>GTMAAAAVVAATVPAQSMGADGASSVHWFRKGLRLHDNPALL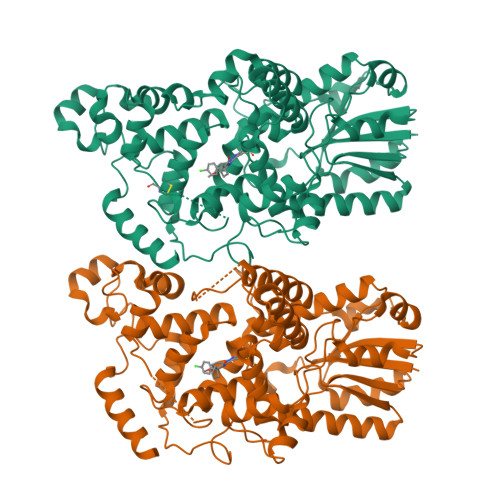AAVRGARCVRCVYILDPWFAASSSVGINRWRFLLQSLEDLDTSLRKLNSRLFVVRGQPADVFPRLFKEWGVTRLTFEYDSEPFGKERDAAIMKMAKEAGVEVVTENSHTLYDLDRIIELNGQKPPLTYKRFQALISRMELPKKPAVAVSSQQMESCRAEIQENHDDTYGVPSLEELGFPTEGLGPAVWQGGETEALARLDKHLERKAWVANYERPRMNANSLLASPTGLSPYLRFGCLSCRLFYYRLWDLYKKVKRNSTPPLSLFGQLLWREFFYTAATNNPRFDRMEGNPICIQIPWDRNPEALAKWAEGKTGFPWIDAIMTQLRQEGWIHHLARHAVACFLTRGDLWVSWESGVRVFDELLLDADFSVNAGSWMWLSCSAFFQQFFHCYCPVGFGRRTDPSGDYIRRYLPKLKGFPSRYIYEPWNAPESVQKAAKCIIGVDYPRPIVNHAETSRLNIERMKQIYQQLSRY[2x]> GPLGSPEFGYWITCCPTCDVDINTWVPFYSTELNKPA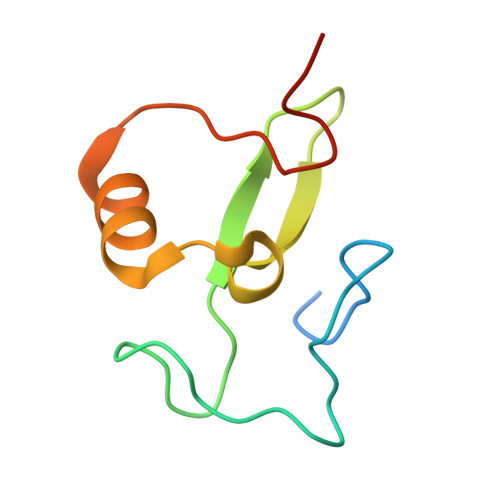MIYCSHGDGHWVHAQCMDLEERTLIHLSEGSNKYYCNEHVQIARA The fungal Bromodomain and Extra‐Terminal (BET) protein Bdf1 is a potential antifungal target against invasive fungal infections. One attractive target is the fungal BET protein Bdf1, a global transcriptional regulator. BET proteins bind chromatin through their two bromodomains (BDs), BD1 and BD2, which specifically recognize histones acetylated on lysines. We show that Bdf1 is essential in C. glabrata, and that inactivation of both Bdf1 BDs induces lethality.

We used a peptide array comprising histone sequences with diverse post‐translational modifications to probe the ligand selectivity of C. glabrata Bdf1 (CgBdf1) BD1 and BD2 (CgBD1 and CgBD2). Like other BET BDs, the two CgBDs displayed weak binding to mono‐acetylated peptides, enhanced binding to di‐ and tri‐acetylated peptides, and strongest binding to a tetra‐acetylated H4 peptide (H4ac4; acetylated on K5, K8, K12 and K16). Substituting a conserved tyrosine implicated in acetyllysine recognition by a phenylalanine (“Y/F” mutations Y166F and Y343F) abolished the interaction with acetylated peptides on the array and in pull‐down assays, demonstrating binding specificity. Crystal structures of CgBD1 and CgBD2 confirmed the expected BD fold (comprising helices Z, A, B and C), allowed comparison with human BET and C. albicans Bdf1 (CaBdf1) BD structures, and revealed details of the ligand binding pockets defined by the ZA and BC loops, including six structurally conserved water molecules. However, a major obstacle to the development of antifungal BET inhibitors is the requirement for a fungal‐selective dual BD inhibitor (a compound that inhibits both Bdf1 BDs with selectivity over human BET BDs). This challenge arises because the ligand binding pockets of Bdf1 BD1 and BD2 are more divergent than those of their orthologous human BET BDs. Structural modeling predicts that CgBD1 would also engage I‐BET151 less intimately than Brd4 BD1, since CgBD1 residues Arg150 and Gln154 point away from the ligand, unlike the corresponding inward‐pointing Trp81 and Gln85 residues of Brd4.

>GAMGIPQHQQKHALMAIKAVKRLKDARPFLQPVDPVALNIPLYFNFIKRPMDLQTIERKLNANAYETPEQITEDFNLMVENSAKFNGPTAVITQMGRNIQAAFEKHMLNMPAKD[2x]>QEVRRGDFVRNWQLVAAVPLFQKLGPAVLVEIVRALRARTVPAGAVICRIGEPGDRMFFVVEGSVSV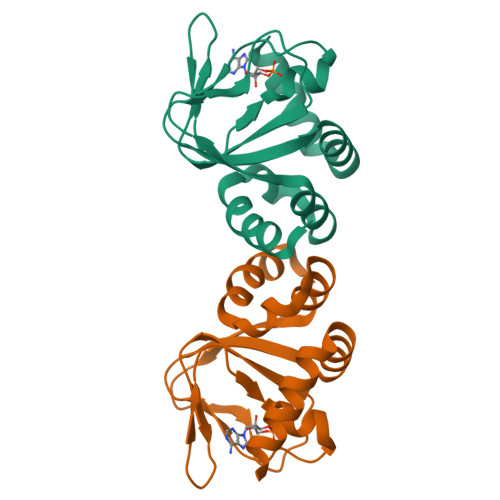ATPNPVELGPGAFFGEMALISGEPESATVSAATTVSLLSLHSADFQMLCSSSPEIAEIFRKTALERRGAAASA[2x]We showed by HPAEC-PAD and LC-FD-MS/MS that RgGH98 is specific for blood group A tetrasaccharide type II (BgA II). As expected from the construct, RgGH98 adopts a modular structure with 3 domains. Structural alignment to homologous GH98 enzymes identified the binding pocket and the general acid catalytic residue as Glu 411, which is present in a cleft in the centre of the Cd. Fragmentation of this species showed that the deoxy-hexose was linked to the hexose at the reducing end, as determined by the characteristic fragments at 431 and 449 Da. Together, the HPAEC-PAD and MS/MS analyses confirmed that BgAtri was released from mucin following RgGH98 hydrolysis of the Galβ1-4GlcNAc glycosidic linkage in BgA II.

We generated an RgGH98 E411A mutant and obtained a complex with the unprocessed carbohydrate following incubation of RgGH98 E411A crystals with BgA II (GalNAcα1–3[Fucα1–2]Galβ1-4GlcNAc). We showed that RgGH98 specificity for BgA is achieved through the precise positioning of amino acid side chains around the BgA GalNAc moiety, as shown in the crystal structure of the complex between RgGH98 E411A and BgA II, principally through Gln 305, Trp 528, and Lys 788. When the complexes with BgAtri (trisaccharide) and BgA II (tetrasaccharide) were overlaid, the GlcNAc residue was found to be very close to Glu 411 at <2 Å in the tetrasaccharide complex. The GlcNAc spatial arrangement is in contrast to the Sp3GH98 complex, in which the GlcNAc residue is pivoted with respect to Gal. It is proposed that Glu 411 adopts a different rotamer in the presence of substrate. As well as bringing the side chain into a position from which a steric clash is avoided, this shift also provides a change in local environment, which may alter residue’s pKa, promoting catalysis. Density for an additional BgA II tetrasaccharide was observed at the C-term domain. Interactions are primarily with the terminal GalNAc of BgA II, specifically with Lys713, Glu734, Glu814, Arg816, Thr817. In the RgGH98 E411A-BgA II complex, 2 metal ions were modelled. The first, a magnesium ion, in the GBLD N-term, coordinated by the side chains of Asp 79, Tyr 84, and Glu 255 and the backbone carbonyls of Leu 76 and Met 254. The second, a calcium ion, in the C-term domain, coordinated by Asp 812, Asn 813, and Gln 846, with additional water models filling the octahedral geometry.

> APPLVNLAEEKDVKVTVGENMDLKNADLLTDGDKYYLQHDATGNKEGNNWENYQEQGTEVTSTAEGKNGVWVQVDLGASYPLEVINLKRQVYDGQATIGNGNPSGQGKRLKGTKISYKNTAIVIGNEEDLSDGQIVYYEGNPTLPDGVKQPENVSKPYEEAMGGQWFYMDYANKNGLGATELGTTKEARYIRVYTENPKGAAVKFMELGIYGYENEQDVQSQDGPRRVIDNEHPMMIATAYSNDVYEIGQEEGPELQGSNTVDGRWNAIPDDLKENNVLLLHTNNLRQFAPDHIGQAYLQAFHEHGLQIAYEQGAPIMLLGLTAAATPENGGTQYNITADMDYGWLDLMYRMYPNMQGVFNTANFWAGIHPPCEGSAKMLEIADRFGGFFVWSDQDHGSTVTNIVSNANMKKALEKHGDAFYLIYKNTSSNQPDDLKTSSFFQGSWLAGYTGGWGMLSDTWAWDKQFSKLWQGAGSYNNWQRLCGEPEALLGMQMMSTYLGGGVIYTFEFPEIVYGTSNTNSPANTHVLTELFRYIVNHPAPSKKEIMEETKAVLYGNVSSDFYSGLSGKPTGFQIYETGRYGIIPVIPTWGTRAEVTKKLIQEADKLGVTPPNVLDVKDKNLSGQAKQKYFKDLYPIEYVGNAFADKWEGTWYLYNNKVNTNEKQHAILPLEGEEESARLKVEMEPHEFMIMNESGDGTAMDITLNNYRVNKDEIIFDNKFGLTWTGDFSPGQTTINGKLSVYKYMDEYNVVNAPEGKLSPEDNELRTTTFELTKLAKEPKVQVVKGQQPDTDGQPQYTEPKVEFNEETGKAVITIQTNGWVDLSITGLEFVYDENAQKIEDE>MENGYTYEDYKNTAEWLLSHTKHRPQVAIICGSGLGGLTDKLTQAQIFDYSEIPNFPRSTVPGHAGRLVFGFLNGRACVMMQGRFHMYEG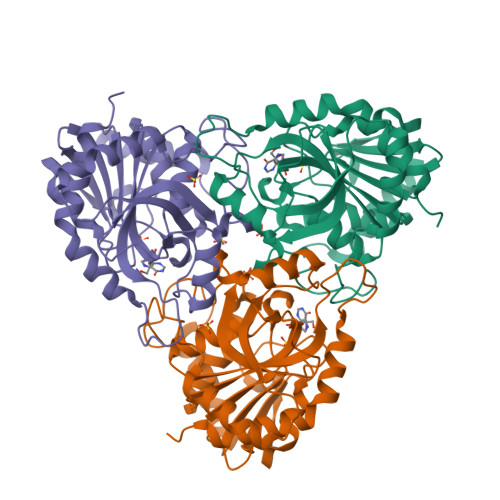YPLWKVTFPVRVFHLLGVDTLVVTNAAGGLNPKFEVGDIMLIRDHINLPGFSGQNPLRGPNDERFGDRFPAMSDAYDRTMRQRALSTWKQMGEQRELQEGTYVMVAGPSFETVAECRVLQKLGADAVGMSTVPEVIVARHCGLRVFGFSLITNKVIMDYESLEKANHEEVLAAGKQAAQKLEQFVSILMASIPLPDKAS[6x]> MSIDSALNWDGEMTVTRFDSKTGAHFVIRLDSTQLGPAAGGTRAAQYSQLADALTDAGKLAGAMTLKMAVSNLPMGGGKSVIALPAPRHSIDPSTWARILRIHAENIDKLSGNYWTGPDVNTNSADMDTLNDTTEFVFGRSLERGGAGSSAFTTAVGVFEAMKATVAHRGLGSLDGLTVLVQGLGAVGGSLASLAAEAGAQLLVADTDTERVAHAVALGHTAVALEDVLSTPCDVFAPCAMGGVITTEVARTLDCSVVAGAANNVIADEAASDILHARGILYAPDFVANAGGAIHLVGREVLGWSESVVHERAVAIGDTLNQVFEISDNDGVTPDEAARTLAGRRAREASTTTATA;> MSIDSALNWDGEMTVTRFDRMTGAHFVIRLDSTQLGPAAGGTRAAQYSQLADALTDAGKLAGAMTLKMAVSNLPMGGGKSVIALPAPRHSIDPSTWARILRIHAENIDKLSGNYWTGPDVNTNSADMDTLNDTTEFVFGRSLERGGAGSSAFTTAVGVFEAMKATVAHRGLGSLDGLTVLVQGLGAVGGSLASLAAEAGAQLLVADTDTERVAHAVALGHTAVALEDVLSTPCDVFAPCAMGGVITTEVARTLDCSVVAGAANNVIADEAASDILHARGILYAPDFVANAGGAIHLVGREVLGWSESVVHERAVAIGDTLNQVFEISDNDGVTPDEAAR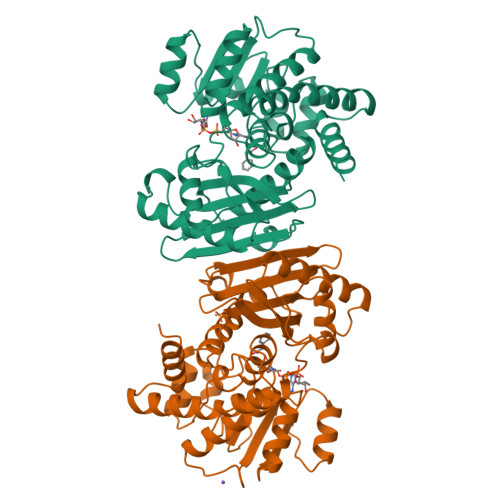TLAGRRAREASTTTATA> MDGVHDLAGVQGFGKVPHTVNADIGPTFHAEWEHLPYSLMFAGVAELGAFSVDEVRYVVERMEPRHYMMTPFYERYVIGVATLMVEKGILTQDELESLAGGPFPLSRP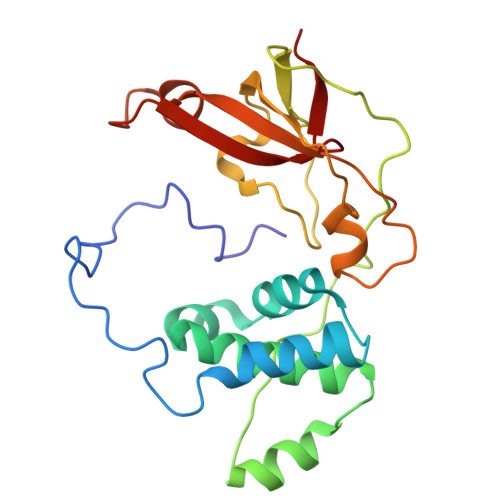SESEGRPAPVETTTFEVGQRVRVRDEYVPGHIRMPAYCRGRVGTISHRTTEKWPFPDAIGHGRNDAGEEPTYHVKFAAEELFGSDTDGGSVVVDLFEGYLEPAA>MPATDTLSLSASEALARRRSVRAFTDRPVDRALLARIFEIAQRAP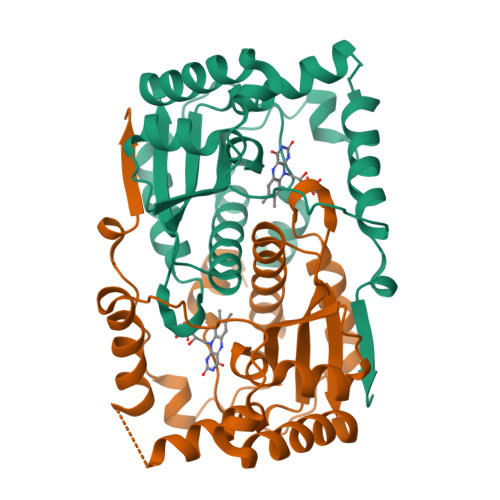SGGNLQPWQATVVTGERWQAVQDAVAARIVMGREGFQPEYDIAPRGLTDPWDSRRFGVGEALYASLGIARDDKAGRIAQFQQNYRGFGAPVMLFLHCSRIMGPPQWADMGMWLQSVMLLLVEHGLASCPQECWAMYGATVRAELGLGDDQILFSGLAIGHADEEAPVNRWPVPRVGLDEVIDWQGFDA[2x]> GPGYQDPARSVRHIAIPAHRGLITDRNGEPLAVSTPVTTLWANPKELMTAKERWPQLAAALGQDTKLFADRIEQNAEREFIYLVRGLTPEQGEGVIALKVPGVYSIEEFRRFYPAGEVVAHAVGFTDVDDRGREGIELAFDEWLAGVPGKRQVLKDRRGRVIKDVQVTKNAKPGKTLALSIDLRLQYLAHRELRNALLENGAKAGSLVIMDVKTGEILAMTNQPTYNPNNRRNLQPAAMRNRAMIDVFEPGSTVKPFSMSAALASGRWKPSDIVDVYPGTLQIGRYTIRDVSRNSRQLDLTGILIKSSNVGISKIAFDIGAESIYSVMQQVGLGQDTGLGFPGERVGNLPNHRKWPKAETATLAYGYGLSVTAIQLAHAYAALANDGKSVPLSMTRVDRVPDGVQVISPEVASTVQGMLQQVVEAQGGVFRAQVPGYHAAGKSGTARKVSVGTKGYRENAYRSLFAGFAPATDPRIAMVVVIDEPSKAGYFGGLVSAPVFSKVMAGALRLMNVPPDNLPTATEQQQVNAAPAKGGRG

β-Lactam antibacterials, that is, penicillins, carbapenems, monobactams, and cephalosporins, target the penicillin-binding protein (PBP) family of transpeptidases. In Gram-negative bacteria, inhibition of high-molecular mass (HMM) class A and class B PBPs (PBP1a/b, PBP2, and PBP3) is typically lethal. We used high-throughput X-ray crystallography to explore reactions of a boron-containing fragment set with the Pseudomonas aeruginosa PBP3 (PaPBP3). Multiple crystal structures reveal that boronic acids react with PBPs to give tricovalently linked complexes bonded to Ser294, Ser349, and Lys484 of PaPBP3; benzoxaboroles react with PaPBP3 via reaction with two nucleophilic serines (Ser294 and Ser349) to give dicovalently linked complexes; and vaborbactam reacts to give a monocovalently linked complex.

The observed binding mode depends on the nature of the boron compound, with vaborbactam reacting monocovalently, benzoxaboroles (3–15) reacting dicovalently, and phenyl boronates (1 and 2) reacting tricovalently. Structures of boronates 1 and 2 with PaPBP3 show the boron atom is sp3-hybridized and tricovalently bonded to Ser294 (the catalytic serine), Ser349 (from the conserved SxN motif), and Lys484 (in the KS(T)G motif). The reaction of Lys484 is notable and may in part reflect a low pKa for this residue. The phenyl rings of 1 and 2 occupy similar, but distinct, regions at the active site. Water occupies the oxyanion hole that is occupied by the β-lactam-derived carbonyl of PBP inhibitors. The tetrazole of 1 makes hydrogen-bonds to the backbone NHs of Gly534 and Gly535 and is positioned to hydrogen bond with the Thr487 and Ser485 side chains. The direct hydrogen-bonds to Gly534 and Gly535 are unusual for PBP3 inhibitors that occupy the carboxylic acid binding pocket, that is, the pocket binding the C-3 penicillin carboxylate. Importantly, structures of 1 and 2 demonstrate the potential for non-acid groups to engage the PBP3 acid binding pocket—optimized binding of these groups may be used to combat point mutation-mediated resistance in this region. However, although the observed densities were weak, in the complexes with 1, 3, and 13, unique conformations of the β5-α11 loop were observed.1-phenyl-3-pyridin-4-yl-~{N}-(pyridin-4-ylmethyl)pyrazole-4-carboxamide | C21 H17 N5 O | 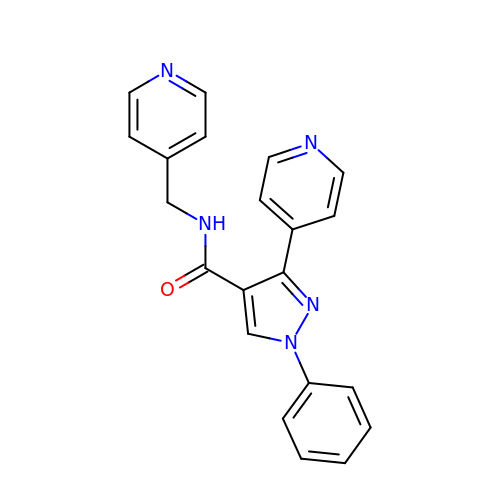IOZGCMLGYOLKER-UHFFFAOYSA-N>AAVMTAEDLKGFEVSVMSWNIDGLDGRSLLTRMKAVAHIVKNVNPDILFLQEVVDRDLAPIDKLQSLYKIYYSNKGCQYY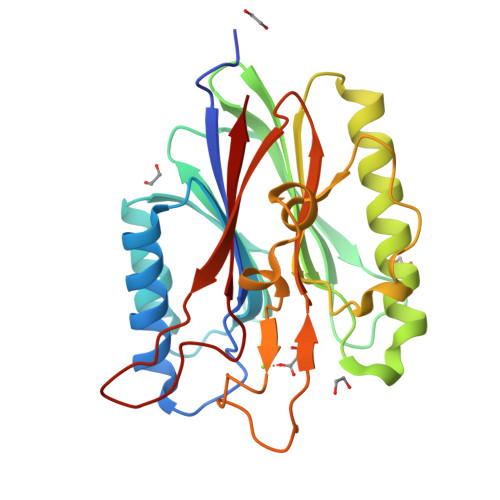TAILVSKMFDVEKHDVIHFQNSGMYRTLQILEGSIGGLKVFLLNTHLESTREHRPQRCAQFGFCMDKVREIIAQNPGALVFFGGDLNLRDEEVSRVPDGVKDAWEAAGSDNKTKFTWDTFKNDNKQGFHGAKMRFDRLYWSGPLDKVKFTLEGRQRIRSCLCFPSDHWAINATFFA[4x]>[2x]SHMLRPVETPTREIKKLDGLWAFSLDRENCGIDQRWWESALQESRAIAVPGSFNDQFADADIRNYAGNVWYQREVFIPKGWAGQRIVLRFDAVTHYGKVWVNNQEVMEHQGGYTPFEADVTPYVIAGKSVRITVCVNNELNWQTIPPGMVITDENGKKKQSYFHDFFNYAGIHRSVMLYTTPNTWVDDITVVTHVAQDCNHASVDWQVVANGDVSVELRDADQQVVATGQGTSGTLQVVNPHLWQPGEGYLYELCVTAKSQTECDIYPLRVGIRSVAVKGEQFLINHKPFYFTGFGRHEDADLRGKGFDNVLMVHDHALMDWIGANSYRTSHYPYAEEMLDWADEHGIVVIDETAAVGFNLSLGIGFEAGNKPKELYSEEAVNGETQQAHLQAIKELIARDKNHPSVVMWSIANEPDTR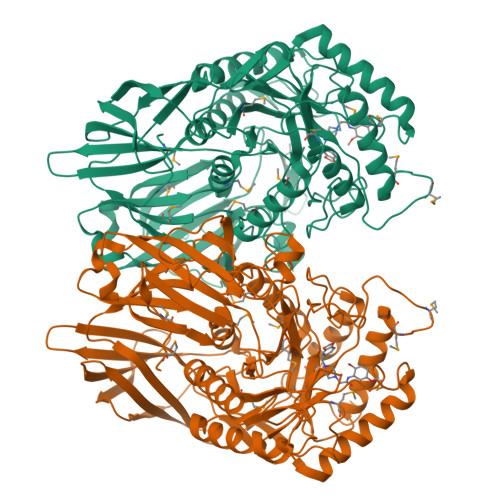PQGAREYFAPLAEATRKLDPTRPITCVNVMFCDAHTDTISDLFDVLCLNRYYGWYVQSGDLETAEKVLEKELLAWQEKLHQPIIITEYGVDTLAGLHSMYTDMWSEEYQCAWLDMYHRVFDRVSAVVGEQVWNFADFATSQGILRVGGNKKGIFTRDRKPKSAAFLLQKRWTGMNFGEKPQQGG>KAGVLKLPIESIHRDKDAPRTYFDEEKLKELSESIKAQGVLQPILVRKDGDGYRIIAGERRWRASQAAGLKEVPAIVRDVTEVQAFELALVENLQRADLNPIEEAEGYKRLVDEFKLTQEQVSVRV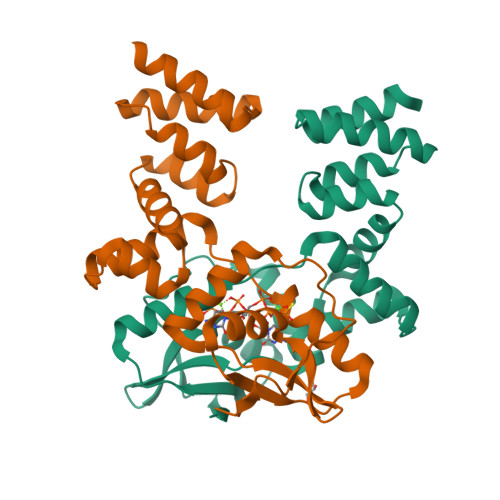GKERSTVANALRLLALPTDVKGMVADGSLSMGHARALLGVPRLPELQNLAKQVADKKLSVRDTERLVQQSRSSGKKDAGKAAPKQS[2x]>GQDMVSPPPPIADEPLTVNTGIYLIECYSLDDKAETFKVNAFLSLSWKDRRLAFDPVRSGVRVKTYEPEAIWIPEIRFVNVENARAADVVDISVSPDGTVQYLERFSARVLSPLDFRRYPFDSQTLHIYLIVRSVDTRNIVLAVDLEKVGKNDDVFLTGWDIESFTAVVKPANFALEDRLESKLDYQLRISRQYFSYIPNIILPMLFILFISWTAFWSTSYEANVTLVVSTLIAHIAFNILVETNLPKTPYMTYTGAIIFMIYLFYFVAVIEVTVQHYLKVESQPARAAS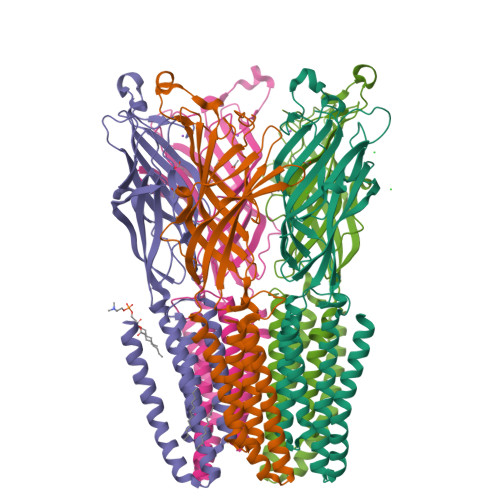ITRASRIAFPVVFLLANIILAFLFFGF[5x]O-NITROPHENOL 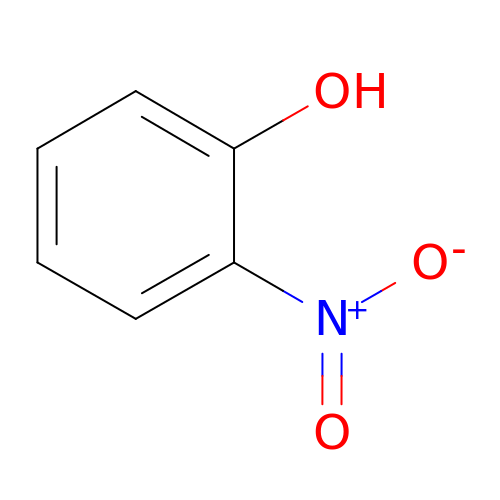| C6 H5 N O3 | IQUPABOKLQSFBK-UHFFFAOYSA-N> GAMGAWKLQTVLEKVRLSRHEISEAAEVVNWVVEHLLRRLQGGESEFKGVALLRTGSYYERVKISAPNQFNVMFKLEVPRIQLEEYCNSGAHYFVKFKRNPGGNPLEQFLEKEILSASKMLSKFRKIIKEEIKNIEDTGVTVERKRRGSPAVTLLISKPKEISVDIILALESKSSWPASTQKGLPISQWLGAKVKNNLKRQPFYLVPKHAKEGSGFQEETWRLSFSHIEKDILKNHGQSKTCCEIDGVKCCRKECLKLMKYLLEQLKKKFGNRRELAKFCSYHVKTAFFHVCTQDPHDNQWHLKNLECCFDNCVA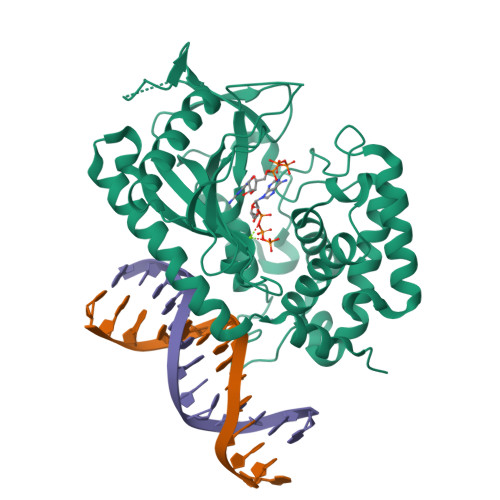YFLQCLKTEQLANYFIPGVNLFSRDLIDKPSKEFLSKQIEYERNNGFPVFW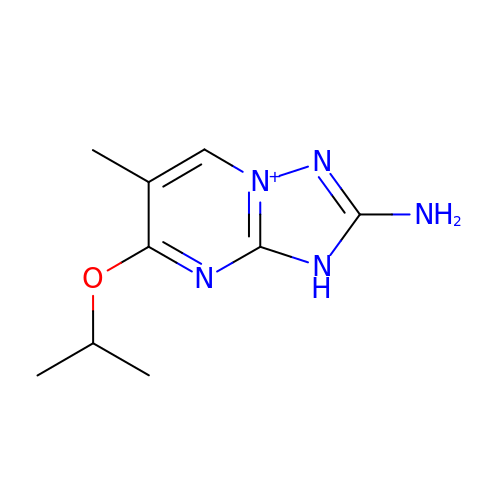2-amino-6-methyl-5-(propan-2-yloxy)-3H-[1,2,4]triazolo[1,5-a]pyrimidin-8-ium | C9 H14 N5 O | FTYINYVODPUDCY-UHFFFAOYSA-O>[2x]ENITQWNLQDNGTEGIQRAMFQRGVNRSLHGIWPEKICTGVPSHLATDTELKAIH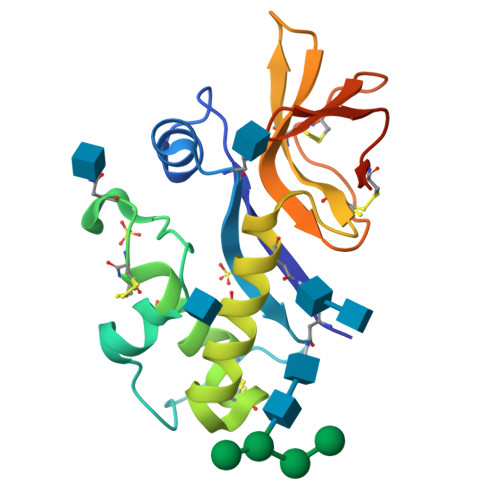GMMDASEKTNYTCCRLQRHEWNKHGWCNWYNIEPWILLMNKTQANLTEGQPLRECAVTCRYDRDSDLNVVTQARDSPTPLTGCKKGKNFSFAGILVQGPCNFEIAVSDVL>[2x]MNNIWWQTKGQGNVHLVLLHGWGLNAEVWRCIDEELSSHFTLHLVDLPGFGRSRGFGALSLADMAEAVLQQAPDKAIWLGWALGGLVASQIALTHPERVQALVTVASSPCFSARDEWPGIKPDVLAGFQQQLSDDFQRTVERFLALQTMGT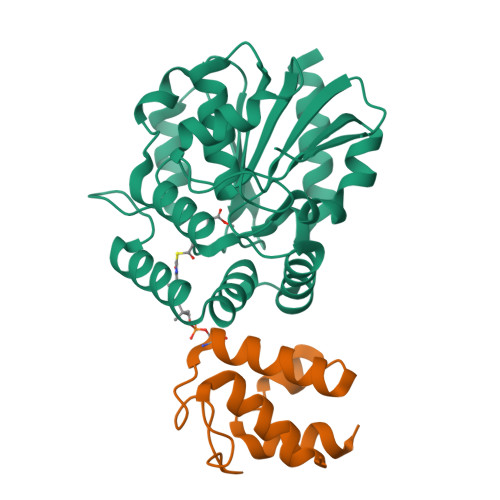ETARQDARALKKTVLALPMPEVDVLNGGLEILKTVDLRQPLQNVSMPFLRLYGYLDGLVPRKVVPMLDKLWPHSESYIFAKAAHAPFISHPAEFCHLLVALKQRVLEHHHHHH;>[2x]STIEERVKKIIGEQLGVKQEEVTNNASFVEDLGADSLDTVELVMALEEEFDTEIPDEEAEKITTVQAAIDYINGHQA>MWSHPQFEKSAMPFVGGAESGDPLGAGRPIGDDECEQYTSSVSLARMLYGGDLAEWVPRVHPKTTIERQQHGPVTFPNASAPTARCVTVVRAPMGSGKTTALIRWLREAIHSPDTSVLVVSCRRSFTQTLATRFAESGLVDFVTYFSSTNYIMNDRPFHRLIVQVESLHRVGPNLLNNYDVLVLDEVMSTLGQLYSPTMQQLGRVDALMLRLLRTCPRIIAMDATANAQLVDFLCGLRGEKNVHVVVGEYAMPGFSARRCLFLPRLGTELLQAALRPPGPPSGPSPDASPDARGATFFGELEARLGGGDNICIFSSTVSFAEIVARFCRQFTDRVLLLHSLTPLGDVTTWGQYRVVIYTTVVTVGLSFDPLHFDGMFAYVKPMNYGPDMVSVYQSLGRVRTLRKGELLIYMDGSGARSEPVFTPMLLNHVVSSCGQWPAQFSQVTNLLCRRFKGRCDASACDTSLGRGSRIYNKFRYKHYFERCTLACLSDSLNILHMLLTLNCIRVRFWGHDDTLTPKDFCLFLRGVHFDALRAQRDLRELRCRDPEASLPAQAAETEEVGLFVEKYLRSDVAPAEIVALMRNLNSLMGRTRFIYLALLEACLRVPMATRSSAIFRRIYDHYATGVIPTINVTGELELVALPPTLNVTPVWELLCLCSTMAARLHWDSAAGGSGRTFGPDDVLDLLTPHYDRYMQLVFELGHCNVTDGLLLSEEAVKRVADALSGCPPRGSVSETDHAVALFKIIWGELFGVQMAKSTQTFPGAGRVKNLTKQTIVGLLDAHHIDHSACRTHRQLYALLMAHKREFAGARFKLRVPAWGRCLRTHSSSANPNADIILEAALSELPTEAWPMMQGAVNFSTL[2x]

At the core of HSV-1 replication initiation is the OBP, a 94 kDa protein encoded by the UL9 gene. As an essential component of the viral replication machinery, OBP integrates multiple critical functions: origin recognition, DNA binding, and ATP-dependent helicase activity. OBP consists of two major functional domains: an N-terminal helicase-like domain (residues 1–535) and a C-terminal origin-binding domain (residues 536–851). The structures reveal a head-to-tail dimer architecture, with DNA binding on one side.

The first structure, representing complex I, shows OBP bound to modified OriS, where the removal of six base pairs from the AT-rich region stabilizes cooperative binding of OBP to OriS but prevents unwinding initiation. Our high-resolution OBP + OriS-6AT structure captures detailed interactions between the conserved R756VKNL motif and its target Box 1 sequence (GTTCGCAC) in the DNA major groove. We observe two distinct types of protein-DNA contacts: sequence-specific base recognition and phosphate backbone interactions. The backbone contacts involve a network of main chain amides: H782 bonds with the D/G23 phosphate, K762 engages the D/T24 phosphate, and both T750 and V757 contact the C/T52 phosphate. Within the RVKNL motif, K758 plays a critical role in sequence specificity through multiple contacts. This key residue makes both backbone and base-specific interactions: its main chain carbonyl recognizes the D/C26 cytosine's amine group, while its side chain reaches deep into the major groove to form hydrogen bonds with both C/G53 guanine's carbonyl and D/G27 guanine's N7. Specifically, substituting D/G27 with thymine in Box 3 would create a steric clash with K758, offering the first structural explanation for how OBP differentially recognizes Box 1 versus Box 3. Additional sequence-specific contacts are mediated by R783, which forms an intricate network of interactions with D/G23 (both carbonyl and N7 positions) and D/T24’s carbonyl group. This precise arrangement explains another aspect of binding site selectivity: substituting D/T24 with cytosine in Box 2 would disrupt these R783-mediated interactions, providing a structural basis for the differential binding affinity between Boxes 1 and 2. We identify multiple basic residues (K793, K802, R810, K746) as well as Q743, Y786, and potentially K780, engaging the DNA phosphate backbone through an elaborate hydrogen bonding network.> PSTLELLKDVHLGLPVPCHDPARLALLSGHYLYYHYGCDGLDDRGWGCGYRTLQTLCSWPGGQSSGVPGLPALQGALEAMGDKPPGFRGSRNWIGCVEASLCLEHFGGPQGRLCHLPRGVGLRGEEERLYSHFTTGGGPVMVGGD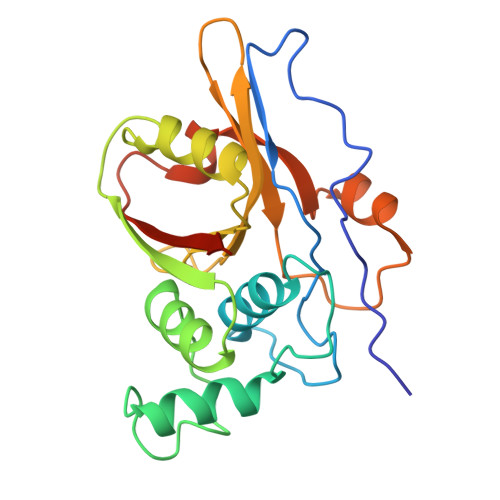ADAQSKALLGICEGPGSEVYVLILDPHYWGTPKNRCELQAAGWVGWQKVKSVFDSNSFYNLCFTRLEHHHHHH> GAMGMTTDEGAKNNEESPTATVAEQGEDITSKKDRGVLKIVKRVGNGEETPMIGDKVYVHYKG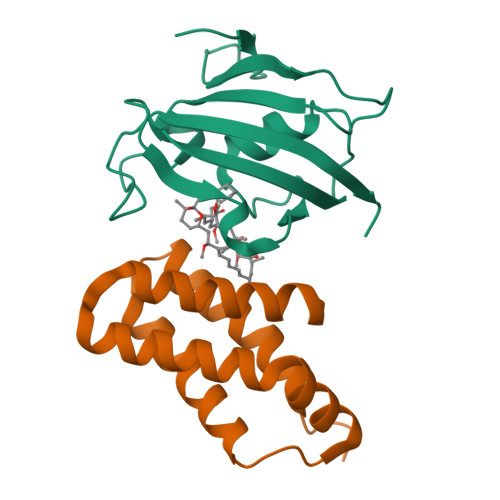KLSNGKKFDSSHDRNEPFVFSLGKGQVIKAWDIGVATMKKGEICHLLCKPEYAYGSAGSLPKIPSNATLFFEIELLDFKGE;> GAMDPEFMEMWHEGLEEASRLYFGERNVKGMFEVLEPLHAMMERGPQTLKETSFNQAYGRDLMEAQEWCRKYMKSGNVKDLTQAWDLYYHVFRRISKQ> 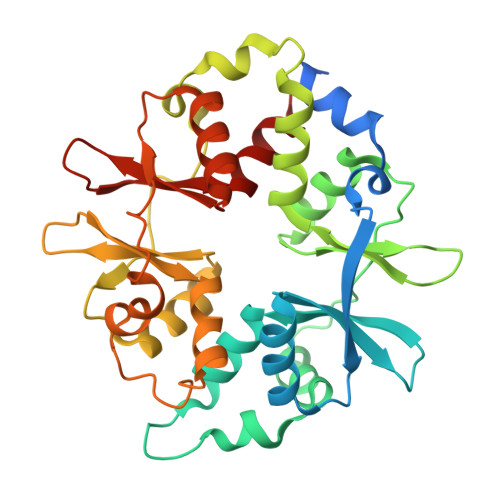METVISSDSSPAVENEHPQETPESNNSVYTSFMKSHRCYDLIPTSSKLVVFDTSLQVKKAFFALVTNGVRAAPLWDSKKQSFVGMLTITDFINILHRYYKSALVQIYELEEHKIETWREVYLQDSFKPLVCISPNASLFDAVSSLIRNKIHRLPVIDPESGNTLYILTHKRILKFLKLFITEFPKPEFMSKSLEELQIGTYANIAMVRTTTPVYVALGIFVQHRVSALPVVDEKGRVVDIYSKFDVINLAAEKTYNNLDVSVTKALQHRSHYFEGVLKCYLHETLETIINRLVEAEVHRLVVVDENDVVKGIVSLSDILQALVLT> MFAWWGRTVYRYRFIVIGVMVALCLGGGVFGLSLGKHVTQSGFYDDGSQSVQASVLGDQVYGRDRSGHIVAIFQAPAGKTVDDPAWSKKVVDELNRFQQDHPDQVLGWAGYLRASQATGMATADKKYTFVSIPLKGDDDDTILNNYKAIAPDLQRLDGGTVKLAGLQPVAEALTGTIATDQRRMEVLALPLVAVVLFFVFGGVIAAGLPVMVGGLCIAGALGIMRFLAIFGPVHYFAQPVVSLIGLGIAIDYGLFIVSRFREEIAEGYDTETAVRRTVITAGRTVTFSAVLIVASAIGLLLFPQGFLKSLTYATIASVMLSAILSITVLPACLGILGKHVDALGVRTLFRVPFLANWKISAAYLNWLADRLQRTKTREEVEAGFWGKLVNRVMKRPVLFAAPIVIIMILLIIPVGKLSLGGISEKYLPPTNSVRQAQE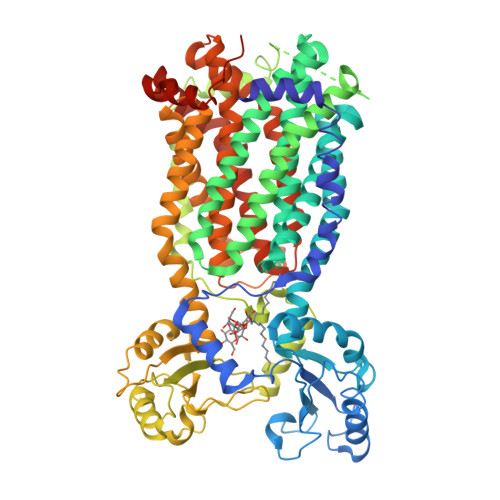EFDKLFPGYRTNPLTLVIQTSNHQPVTDAQIADIRSKAMAIGGFIEPDNDPANMWQERAYAVGASKDPSVRVLQNGLINPADASKKLTELRAITPPKGITVLVGGTPALELDSIHGLFAKMPLMVVILLTTTIVLMFLAFGSVVLPIKATLMSALTLGSTMGILTWIFVDGHFSKWLNFTPTPLTAPVIGLIIALVFGLSTDYEVFLVSRMVEARERGMSTQEAIRIGTAATGRIITAAALIVAVVAGAFVFSDLVMMKYLAFGLMAALLLDATVVRMFLVPSVMKLLGDDCWWAPRWARRLQTRIGLGEIHLPDGSENLYFQ> MSSAFSGLKIPELSVDPAEVFKSDNPQLVSVLLDEFELQEQRPFFSGLIPEKQINIALKKSPQLKKLACHLLEAYEINGRRWKHADRRRVLEKAIRLLEKVSNELKGDIQKLENNVKESGKDSEELNKTREKHGEILADMGRAYLHRAKIIRPKGFTIPAKKKESLRKALDFCKEAKARHLAGLVGLEMDRCDMSDFDSENSLEKLLRDATTGVSLSKDQYYSNEYRKAEYYQMCIRLAEIEEDKHGATDEGSENNRYKRLEGILGPKKSQGKKKGKKNKKKKGTNSKSALEKIMAFEKFKVAVYLGEGKEKTHWNDFSEFLMRYPFSHPSWEDSVRFLRRLYKKGNDKWRELSVALWEIAKKNSAKTSSIHLRWYWSRQRDLYDLAFLSALEQADIAEDESVRQEKLRLAAKVADSAKNRPALTWQAMEQMADKDEALKKEIENYAQALGGGYIEQFEKTELPKNTNPQDDIPDDLKTSGLVVQFYLVHLKDYENGYALIYDGKTKKWSCEMFNFFPIWEKYLQWQSVYFDLPANQKEESADQLKALCLELGRHLYFLFDFEENRKAHEKNQDTAKENWDMLFIPHDFLHRVPIHGAIKKNGTNILLKKFNCTYFPTLPNASITPESPKSDNVAELIEYFSEHEKDYSEYFDKIEHIFDKKNRAATSQDLLDAAISPPRTLTIYCHGQSDVNNPFYSRLLLKDKLELIKLATLQEHYSGTHIFLGACETDLMPPLSAPLDEQLSMAAMFLQKGVGSVLGTLWEAYPRAVKDIVKNILSADDTQYFEKLFSLKKKISVNQKKSLYYYLCFKLYRSFDQIGKE;> MGSSHHHHHHSQDPMQHIIPLTITFLESFRVIEWHKSSDRNSLRFLRGYAYARWHRSLKNNKGRPYITGTLVRSAIIRAAEELLWLNDGNYKGAICCPGEFNGSNAKVFREGKARRLRRRQTLTWPTKCACHEKEPCPFCLLLGRYEKSSKTSKSPVLNNVNFSNFNVLGKEKEFLNIEDVADMRVVNRVDQQSGKAEDFFNIWEITDGAWKIFRGEIQVSDKGWSDEENFSKFLTLLKGASVLVDKISGGLCYLTLDKPELAELPAVKTEKDVLEPGDDASVLEISRPPYWNNMLNLAGTISEAFEREDKLVHLRLFADTVRELRRSDIETLDLPKGHADRLGKPSDHFIWDIEINKKVKLRNWLFWIFNEFRDTYAYFDWRTFCEALGQALYLEAKKQVPNQFSSERPVGATPAMEVKTPEHDPGRAAQGPRYEWLIKGELVSQTPFFFGWSTEADNREHTNLKLLAARDGRLRLPLSVLRGILRRDIKVVLDNKCRAELAMKQPCSCPVCNLMKKITIRDSFSSNYAEPPKIRHKIRLDPKSGTVAKGALFDSEVGPRGVVFPFELRLRSADDTLPQALKTVFSWWQQGTVSFSGDAGTGKGIFCLRNLKSIRWDLKTEMDKYAATLGGRKTPVGKWDKCHIPDDKTYPWVKETVEISVCSPFITKDPVNSLIDSAGYDAICYTTVDLEKSENINSLPESEISLLFEMFDLQYPMSYLFPNKDIYLLKGESFRGMLRTAVGRGENLLLREHEDCSCTLCRIFGNEHNAGKIRVEDFIIQGEPRTKLVDRVAIDRFTAGAKDKFKFDAAPIVGTPTNKLKFRGNIWIHRDLDGLACESLKLALEDIENGLYPFGGLGNAGFGWVNYNPLSHPAQEENKADFSLTKKMELNWSMKELSTDKIYWPHYFLPFGKKVLREKTPPSHACIDENEDSELYSGKIVCTLETRTPLIIPDSEFQGEEHKSYDFFNLNGELCIPGSEIRGMISSVFEALTNSCMRIFDEKKRLSWRMNPNKKDKKNNNRRELDDFIPGRVTNDRKMEEMKEYRYPFYDQAITANDKQNKYFDQWEATIELTDESLEKLKAEKILQSVLDALRPLTKKKEKYKNTETFVFDLKKFIGKIDDNQQMISEALERGKVRLTGNSLKQISKTKKIPRQILN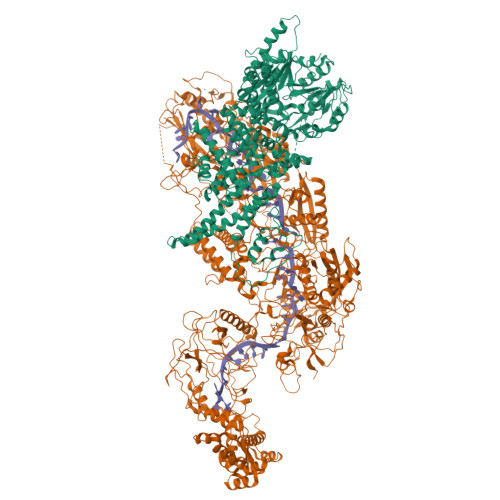QLKGLKDNTYENREQFISVLKTTVRGINDEQISLILDNIDEDVRLTDLSLTKIRKAKVPQTLVDMLADLKKDEPYKNEKEFLSEFKKKMGEIIGLILKHAAKTGGDVPRYNHPTPTDKMLLSLAAYNRNHKHENGKAEYRIVKPKHNLKVDFMFAVTPFENPFKGYNPAAVVEEPVGGYLKVSGPNKIEKVKKVNPNSVSVRDDKNQEIIHNGVYLRKITVANAKSKNKLRERLVPEFAWYDKDSEAAYAMTKRCERVFVEIGAKPIPIQPSAREKFKILTQEYQKNAKQQKTPEAFQTILPKDGELRPGDLVYFREDKKTNTVTDIIPVRISRTVDDEVLARKIPDDVGDVRPCVREILDKEKQKEIADAGVKEVFQHHPDGLCPACSLFGTTFYKGRIAFGFAFHKDKDPELANNGKHITLPLLERPRPTWSMPKKESRVPGRKFYVHHQGWERVIKHSNLDESDPNATKQTVNNRSVQAIKEEQKFQFEVRFENLREWELGLLVYVLQLEPQFAHKLGMGKALGFGSVRIRVGEIHSGPKELDESRLVSSAMKKMEEIWDRDKNVLEKLFRLLYFNESKDIKVRYPKLQKEKEEEEEESGYMELAKEEYQPEQRRNKLTNPWEGWGNILKKPAILI>[2x]MSSGKKP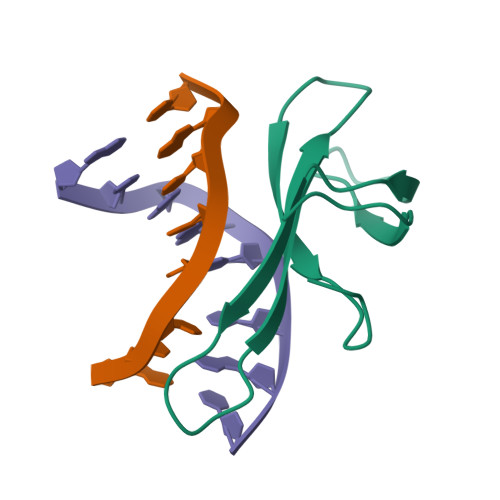VKVKTPAGKEAELVPEKVWAVAPKGRKGVKIGLFKDPETGKYFRHKLPDDYPI>[2x]MNAIADVQSSRDLRNLPINQVGIKDLRFPITLKTAEGTQSTVARLTMTVYLPAEQKGTHMSRFVALMEQHTEVLDFAQLHRLTAEMVALLDSRAGKISVSFPFFRKKTAPVSGIRSLLDYDVSLTGEMKDGAYGHSMKVMIPVTSLCPCSKEISQYGAH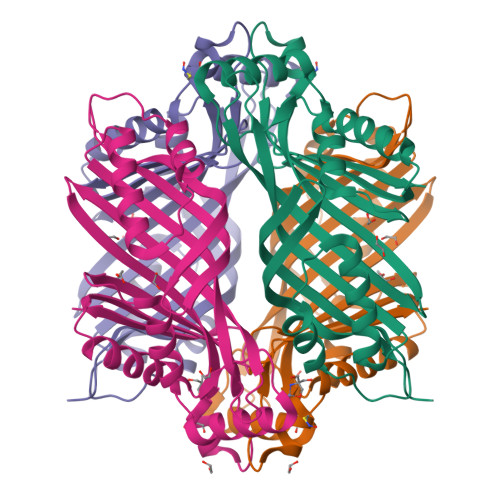NQRSHVTVSLTSDAEVGIEEVIDYVETQASCQLYGLLKRPDEKYVTEKAYENPKFVEDMVRDVATSLIADKRIKSFVVESENFESIHNHSAYAYIAYP>[2x]MSLSGVSHVSLTVRDLDISCRWYTEILDWKELVRGRGDTTSFAHGV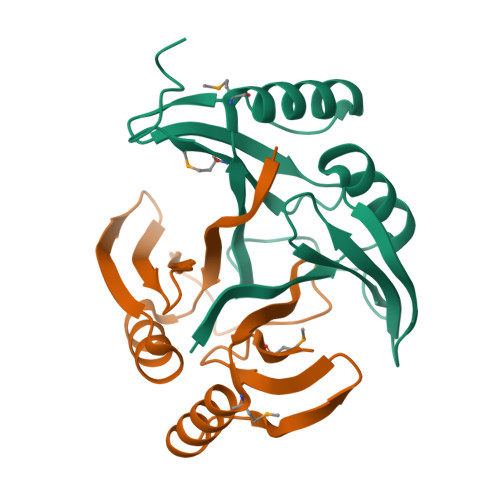LPGGLSIVLREHDGGGTDLFDETRPGLDHLSFSVESMTDLDVLEERLAKAGAAFTPTQELPFGWILAFRDADNIALEAMLGREGHHHHHH>HHHHHHSSGLVPRGSHMAGLGNVTGAVASGDSLTLTLDNGTSASDILELDVLSEELLRVDYRPSGAAPSPSTPMIDPDASWDAVGATIDTSGDPIVVTTPRMRIEIARTPARMTIKKADGTTLLWEPASGGVFEDGVRFQRGSTDNIYGIRSFNAQEDVGGLLRNSSDHPAHAGQQGDAGGPFMWSTAGYGVLVDSDGGYPYTDTTGKLEFYYGGTPTEGRRYTKTNVEYYIMVGEPKEIMASYAQVTGTAPMLPKWSLGFMNFEWGIDQDELEAHVDGYRARNIPIDAFALDYDWMDYGEDNYGEFRWNTDNFPDAATTQLKEDMEAEGIRLIGIRKPRIITRDFANQRTQQYYDADSNGYFYPGHNEYTDYFIPVTVRSFDPYQQASRDWWWQHSIDAFDKGIVGWWNDETDKVDSGSAQYWFGNFSTGFTSQAMYDGQRDYTNDGVRVWQTARSYYPGAQRYATTLWSGDIGTQFYKGELFNWAPGMQEQPRIMLSSANLGQPKWGMDTGGFNSLGGAS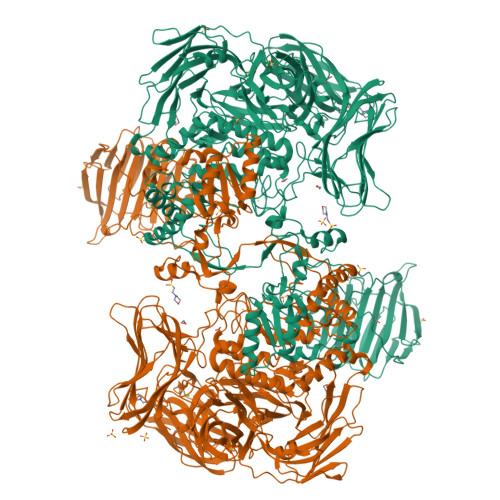GPNPSPELYTRWMQFGAFTPVFRVHGNYNQQRQPWLYGATAEEASKAVMHTRYSLLPYMYAYEREASETGLGLIKPLLFDYPNDPQAADYTEAWMFGDWLLVSPVLGEAQHSKQIYLPAGTWIDYHRGQTYSGGQTIHYPVNADTWTDVPLFVKQGAIIPNQQVLDYVDQQSVTTVNVDIFPSASETSFTYYEDDGSSYDYESGSSFEQRLAAQDLSSSVRVEVGAGSGSYTPDVQHYVLKIHGRAGSAVTAGGSALTGYGDLQALQAASGSGWASGRDIYGDVTYVKLPAASGSATVVEVSGSAPSAATHAIYEVEDASRSGATPTTRAGINTNHSGYSGSGFVDKLDVPGAAVTVYANAPVSGDYPVELRYANGSGSAKTLSVYVNAARVQQLSLADTGAWSQWGTQTTTLPLTAGQNIITYKYDSDAGDTGGVNLDYIRVPFAPTQAEYAAESAKLWGGAGTSQDHWFYKGAAFVDNLTGVGAEASFDVYAPSAGTYNLSLRYANGTGSTKTLSAIVNGGAASTVTLTSPGMNWNLWNEHTMTATLTAGRNTISFRRNSGNSGNVNLDRLAVSASAITTLASERNLLDNGDFERDTTYNSNWTQWQPSGQPSAFGIDSGNALHPPEGPARRNQRAYFHSDNAYQQSIHQVVDVPVNNATYRLEAKVRMKNTTPTTARAEVQGHGGSPIYANISNDGVWKTIVIDNINVTSGSVDVGFYVDSPGYTTLHIDEVTLTRAP[2x]> MGHHHHHHHHHHSSGENLYFQGHMKAKNRKTRKFEPLTFVFSFLLLVLFLFIFLTLSNMIFEQITEDFSGLVKAAGNRSVISSIFLSLYAGFLATLLALLLGAPTGYILARFDFPGKRLVESIIDVPVVVPHTVAGIALLTVFGSRGLIGEPLESYIQFRDALPGIVVAMLFVSMPYLANSAREGFKSVDPRLENAARSLGAPLWKAFFFVTLPLSARYLLIGSVMTWARAISEFGAVVILAYYPMVGPTLIYDRFISYGL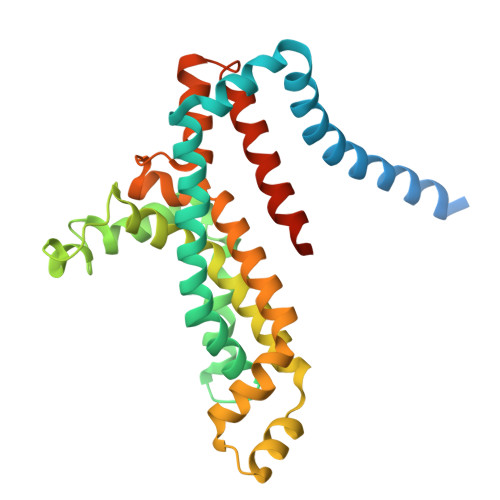SASRPIAVLLILVTLSIFLVIRTLSAGWSIYDRD> APLVHHHHHHALDENLYFQGALATTLDEADEAGKRIFGPRVGNELCEVKHVLDLCRIRESVSEELLQLEAKRQELNSEIAKLNLKIEACKKSIENAKQDLLQLKNVISQTEHSYKELMAQNQPKLSLPIRLLPEKDDAGLPPPKATRGCRLHNCFDYSRCPLTSGFPVYVYDSDQFVFGSYLDPLVKQAFQATARANVYVTENADIACLYVILVGEMQEPVVLRPAELEKQLYSLPHWRTDGHNHVIINLSRKSDTQNLLYNVSTGRAMVAQSTFYTVQYRPGFDLVVSPLVHAMSEPNFMEIPPQVPVKRKYLFTFQGEKIESLRSSLQEARSFEEEMEGDPPADYDDRIIATLKAVQDSKLDQVLVEFTCKNQPKPSLPTEWALCGEREDRLELLKLSTFALIITPGDPRLVISSGCATRLFEALEVGAVPVVLGEQVQLPYQDMLQWNEAALVVPKPRVTEVHFLLRSLSDSDLLAMRRQGRFLWET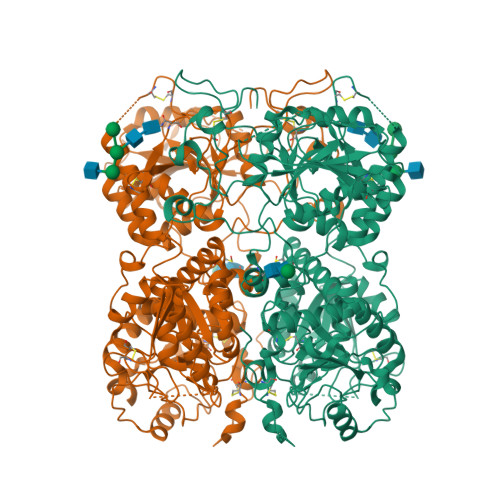YFSTADSIFNTVLAMIRTRIQIPAAPIREEAAAEIPHRSGKAAGTDPNMADNGDLDLGPVETEPPYASPRYLRNFTLTVTDFYRSWNCAPGPFHLFPHTPFDPVLPSEAKFLGSGTGFRPIGGGAGGSGKEFQAALGGNVPREQFTVVMLTYEREEVLMNSLERLNGLPYLNKVVVVWNSPKLPSEDLLWPDIGVPIMVVRTEKNSLNNRFLPWNEIETEAILSIDDDAHLRHDEIMFGFRVWREARDRIVGFPGRYHAWDIPHQSWLYNSNYSCELSMVLTGAAFFHKYYAYLYSYVMPQAIRDMVDEYINCEDIAMNFLVSHITRKPPIKVTSRWTFRCPGCPQALSHDDSHFHERHKCINFFVKVYGYMPLLYTQFRVDSVLFKTRLPHDKTKCFKFI> GSRFVVEKNNLKVTSPDSIKGIYECAIGNFGVPQYGGTLVGTVVYPKSNQKACKSYSDFDISFKS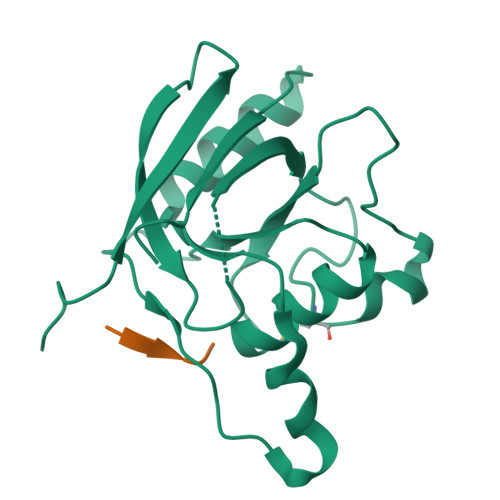KPGRLPTFVLIDRGDCYFTLKAWIAQQAGAAAILVADSKAEPLITMDTPEEDKSDADYLQNITIPSALITKTLGDSIKSALSGGDMVNMKLDWTESVPHP;> XSDRFV>QENRLLNESESSSQGLLGYYFSDLNFQAPMVVTSSTTGDLSIPSSELENIPSENQYFQSAIWSGFIKVKKSDEYTFATSADNHVTMWVDDQEVINKASNSNKIRLEKGRLYQIKIQYQREDPTEKGLDFKLYWTDSQNKKEVISSDNLQLPELKQKSSNSLEVLFQGSTSAGPTVPDRDNDGIPDSLEVEGYTVDVKNKRTFLSPWISNIHEKKGLTKYKSSPEKWSTASDPYSDFEKVTGRIDGNVSPEANHPLVAAYPIVHVDMENIILSKNEDQSTQNTDSQTRTISKNTSTSRTHTSEVHGNAEVHASFFDIGGSVSAGFSNSNSSTVAIDHSLSLAGERTWAETMGLNTADTARLNANIRYVNTGTAPIYNVLPTTSLVLGKNQTLATIKAKENQLSQ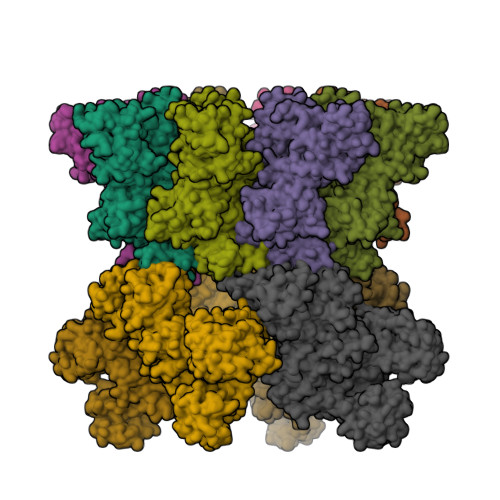ILAPNNYYPSKNLAPIALNAQDDFSSTPITMNYNQFLELEKTKQLRLDTDQVYGNIATYNFENGRVRVDTGSNWSEVLPQIQETTARIIFNGKDLNLVERRIAAVNPSDPLETTKPDMTLKEALKIAFGFNEPNGNLQYQGKDITEFDFNFDQQTSQNIKNQLAELNATNIYTVLDKIKLNAKMNILIRDKRFHYDRNNIAVGADESVVKEAHREVINSSTEGLLLNIDKDIRKILSGYIVEIEDTEGLKEVINDRYDMLNISSLRQDGKTFIDFKKYNDKLPLYISNPNYKVNVYAVTKENTIINPSENGDTSTNGIKKILIFSKKGYEIG[4x];>[4x]QENRLLNESESSSQGLLGYYFSDLNFQAPMVVTSSTTGDLSIPSSELENIPSENQYFQSAIWSGFIKVKKSDEYTFATSADNHVTMWVDDQEVINKASNSNKIRLEKGRLYQIKIQYQRENPTEKGLDFKLYWTDSQNKKEVISSDNLQLPELKQKSSNSLEVLFQGSTSAGPTVPDRDNDGIPDSLEVEGYTVDVKNKRTFLSPWISNIHEKKGLTKYKSSPEKWSTASDPYSDFEKVTGRIDKNVSPEARHPLVAAYPIVHVDMENIILSKNEDQSTQNTDSQTRTISKNTSTSRTHTSEVHGNAEVHASFFDIGGSVSAGFSNSNSSTVAIDHSLSLAGERTWAETMGLNTADTARLNANIRYVNTGTAPIYNVLPTTSLVLGKNQTLATIKAKENQLSQILAPNNYYPSKNLAPIALNAQDDFSSTPITMNYNQFLELEKTKQLRLDTDQVYGNIATYNFENGRVRVDTGSNWSEVLPQIQETTARIIFNGKDLNLVERRIAAVNPSKPLETTKPDMTLKEALKIAFGFNEPNGNLQYQGKDITEFDFNFDQQTSQNIKNQLAELNATNIYTVLDKIKLNAKMNILIRDKRFHYDRNNIAVGADESVVKEAHREVINSSTEGLLLNIDKDIRKILSGYIVEIEDTEGLKEVINDRYDMLNISSLRQDGKTFIDFKKYNDKLPLYISNPNYKVNVYAVTKENTIINPSENGDTSTNGIKKILIFSKKGYEIG;>[4x]AGGHGDVGMHVKEKEKNKDENKRKDEERNKTQEEHLKEIMKHIVKIEVKGEEAVKKEAAEKLLEKVPSDVLEMYKAIGGKIYIVDGDITKHISLEALSEDKKKIKDIYGKDALLHEHYVYAKEGYEPVLVIQSSEDYVENTEKALNVYYEIGKILSRDILSKINQPYQKFLDVLNTIKNASDSDGQDLLFTNQLKEHPTDFSVEFLEQNSNEVQEVFAKAFAYYIEPQHRDVLQLYAPEAFNYMDKFNEQEINLSLEELKDQRMLSRYEKWEKIKQHYQHWSDSLSEEGRGLLKKLQIPIEPKKDDIIHSLSQEEKELLKRIQIDSSDFLSTEEKEFLKKLQIDIRDSLSEEEKELLNRIQVDSSNPLSEKEKEFLKKLKLDIQPYDINQRLQDTGGLIDSPSINLDVRKQYKRDIQNIDALLHQSIGSTLYNKIYLYENMNINNLTATLGADLVDSTDNTKINRGIFNEFKKNFKYSISSNYMIVDINERPALDNERLKWRIQLSPDTRAGYLENGKLILQRNIGLEIKDVQIIKQSEKEYIRIDAKVVPKSKIDTKIQEAQLNINQEWNKALGLPKYTKLITFNVHNRYASNIVESAYLILNEWKNNIQSDLIKKVTNYLVDGNGRFVFTDITLPNIAEQYTHQDEIYEQVHSKGLYVPESRSILLHGPSKGVELRNDSEGFIHEFGHAVDDYAGYLLDKNQSDLVTNSKKFIDIFKEEGSNLTSYGRTNEAEFFAEAFRLMHSTDHAERLKVQKNAPKTFQFINDQIKFIINS> MADTRFPDHAIWTHLDLTSALSVKDPTLLRIKIVPVQPFIANSRKQLDLWASSHLLSMLMYKALEVIVDKFGPEHVIYPSLRDQPFFLKFYLGENIGDEILVANLPNKALAIVSGKEAEKIEEEIKKRIRDFLLQLYREAVDWAVENGVVKVDRSEKDSMLKEAYLKIVREYFTVSITWVSLSEKEDIYQVTENAGLSDEDVKKWLKFAEKKENSRVLERIAIYPLLVKILDSLGERKVTEERFEKSEQLKGWKCHVCGENLAIFGDMYDHDNLKSLWLDEEPLCPMCLIKRYYPVWIRSKTGQKIRFESVVDVALLYKNWRKIFDEKYGKDLVSKAREVSEDFVKDNMLVDSDLYYSSTWESGLSKKLKNKKEIDEEKVKEVVDFLNAAYKEIGNPPKYYAILVMDGDDMGKVISGEVLGEISTRIHPNIRDYVEIPEAKYYSTPQVHVAISQALANFSIREVRSVVKDEGLLIYAGGDDVLAILPVDKALEVAYKIRKEFGKSFENGSLLPGWKLSAGILIVHYKHP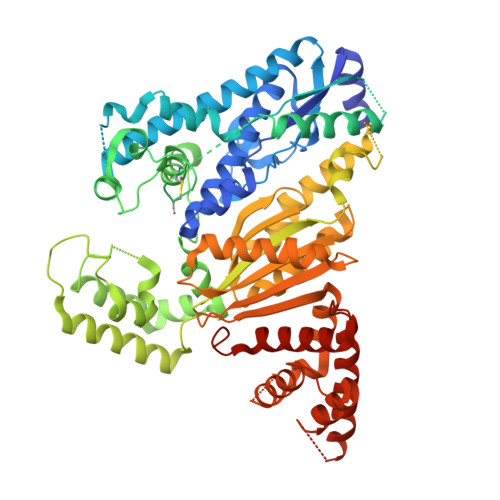LYDALEKARDLLNNKAKNVPGKDTLAIGLLKRSGSYYISLVGWELIRVFYNSELRKKLLEEKGGVGKRFIYHVLREVDTWPKVGIDEMLKFEVIRHIRGRNKEETKELREKIYGEIKDLLEHVRGNNEVEKVRGLFTFLKIITDAEVFPLEHHHHHH>MNQTLLSSFGTPFERVENALAALREGRGVMVLDDEDRENEGDMIFPAETMTVEQMALTIRHGSGIVCLCITEDRRKQLDLPMMVENNTSAYGTGFTVTIEAAEGVTTSVSAADRITTVRAAIADGAKPSDLNRPGHVFPLRAQAGGVLTRGGHTEATIDLMTLA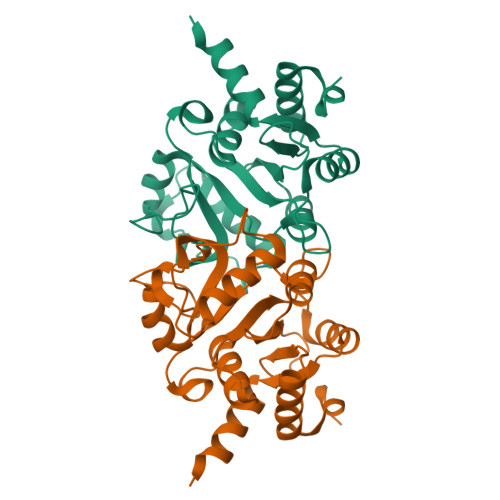GFKPAGVLCELTNDDGTMARAPECIEFANKHNMALVTIEDLVAYRQAHERKASGSSHHHHHH[3x]> MAPPVSERGLKSVVWRKIKTAVFDDCRKEGEWKIMLLDEFTTKLLSSCCKMTDLLEEGITVIENIYKNREPVRQMKALYFISPTPKSVDCFLRDFGSKSEKKYKAAYIYFTDFCPDSLFNKIKASCSKSIRRCKEINISFIPQESQVYTLDVPDAFYYCYSPDPSNASRKEVVMEAMAEQIVTVCATLDENPGVRYKSKPLDNASKLAQLVEKKLEDYYKIDEKGLIKGKTQSQLLIIDRGFDPVSTVLHELTFQAMAYDLLPIENDTYKYKTDGKEKEAVLEEDDDLWVRVRHRHIAVVLEEIPKLMKEISSTKKATEGKTSLSALTQLMKKMPHFRKQISKQVVHLNLAEDCMNKFKLNIEKLCKTEQDLALGTDAEGQRVKDSMLVLLPVLLNKNHDNCDKIRAVLLYIFGINGTTEENLDRLIHNVKIEDDSDMIRNWSHLGVPIVPPSQQAK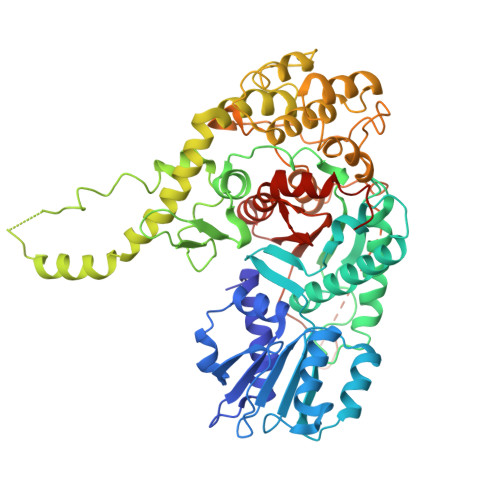PLRKDRSAEETFQLSRWTPFIKDIMEDAIDNRLDSKEWPYCSRCPAVWNGSGAVSARQKPRTNYLELDRKNGSRLIIFVIGGITYSEMRCAYEVSQAHKSCEVIIGSTHILTPRKLLDDIKMLNKSKDKVSFKDE 6-mercaptopyridine-2,3-dicarboxylic acid | C7 H5 N O4 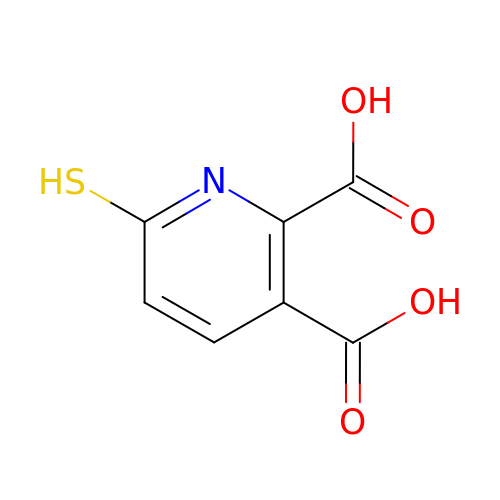S | BQRFMKROEPDXOO-UHFFFAOYSA-N> MRGSHHHHHHGSSHANINAFKEA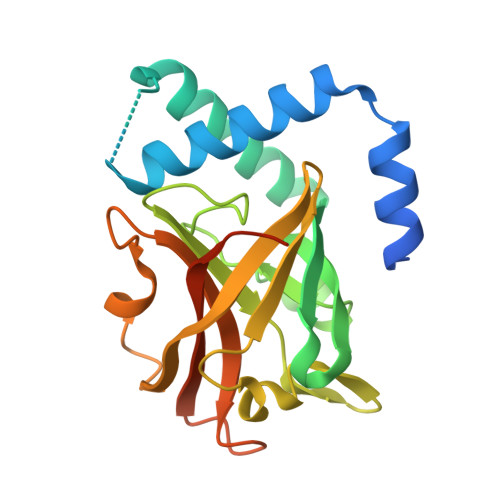VTKIDRVEINRRLELAYAYNASIAGAKTNGEYPALKDPYSAEQKQAGVVEYARMLEVKEQIGHVIIPRINQDIPIYAGSAEENLQRGVGHLEGTSLPVGGESTHAVLTAHRGLPTAKLFTNLDKVTVGDRFYIEHIGGKIAYQVDQIKVIAPDQLEDLYVIQGEDHVTLLTCTPYMINSHRLLVRGKRIPYVEKTVQKDSKTFRQQQ>[2x]GRKKIQ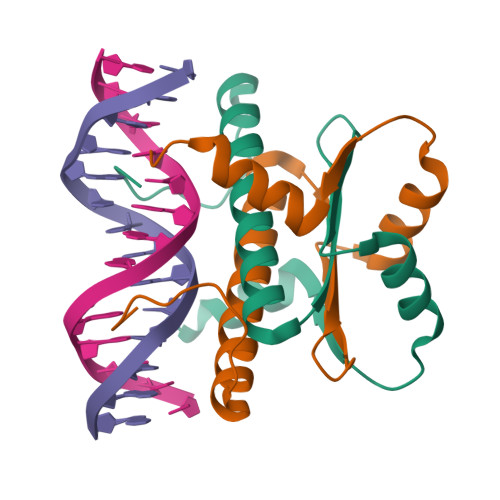IQRITDERNRQVTFTKRKFGLMKKAYELSVLCDCEIALIIFNHSNKLFQYASTDMDKVLLKYTEYNEPHESRTNADIIETLRKKGFN> GALSPGGTKQKYKEVVDIEAQRRLNDLAREARIRRAQQAVLRKELIATSTNVIKSEISLRILASECHLTLNGIVEAEAQYKMGGLPKSRLPKIKH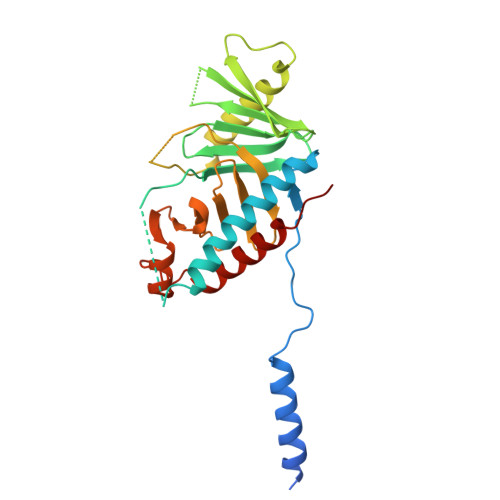PMIVTKWVDYSNKHGFSYQLSTEDIGVLFNNGTTVLRLADAEEFWYISYDDREGWVASHYLLSEKPRELSRHLEVVDFFAKYMKANLSRVSTFGREEYHKDDVFLRRYTRYKPFVMFELSDGTFQFNFKDHHKMAISDGGKLVTYISPSHESTTYPLVEVLKYGEIPGYPESNFREKLTLIKEGLKQKSTIVTVD Class I histone deacetylases (HDACs 1–3) are essential regulators of gene expression. The enzymes are recruited to chromatin as part of large multi-protein complexes that control the acetylation state of histones and other chromatin-associated factors. In the MiDAC complex, the large ELM2-SANT protein MIDEAS (1045 aa), recruits HDAC1 or 2. In conclusion, our structural and functional studies of the MiDAC complex reveal a striking molecular machine whose architecture appears to have evolved to facilitate processive chromatin deacetylation.

For the tetramer, 63,222 particles were included in the final 4.5-Å map with D2 symmetry applied. The tetrameric complex clearly contains a dimer of the dimeric complexes with no obvious structural perturbations. The arrangement is such that the DNTTIP1 dimerisation domains are symmetrically juxtaposed, but do not directly interact. The two S-shaped dimers are rotated 180° with respect to each other with the four HDAC subunits positioned at the periphery of the tetramer, which results in a striking three-dimensional X-shaped complex. This three-dimensional X-shape of the tetrameric complex positions the active sites of the four HDACs at the extremities of the complex. The tetramerisation interface between the two dimers is mediated by interactions between the SANT domains. Residues Lys849, Tyr874 and Val878 contribute to the interface between the two neighbouring SANT domains. Interestingly, Lys839 and Lys843 appear to be in a position to interact with the inositol phosphate that is bound to the neighbouring dimer, although there is no apparent density for the side chains. This may explain why it was only possible to obtain a high-resolution map of the tetramer in the presence of inositol phosphate (7.7 Å vs 4.5 Å). Given the overall size of the MiDAC complex and the outward-facing HDAC active sites at the complex extremities, it is likely that MiDAC is able to simultaneously target multiple nucleosomes.

>MGATGDAEQPRGPSGAERGGLELGDAGAAGQLVLTNPWNIMIKHRQVQRRGRRSQMTTSFTDPAISMDLLRAVLQPSINEEIQTVFNKYMKFFQKAALNVRDNVGEEVDAEQLIQEACRSCLEQAKLLFS[4x];>[4x]MAQTQGTRRKVCYYYDGDVGNYYYGQGHPMKPHRIRMTHNLLLNYGLYRKMEIYRPHKANAEEMTKYHSDDYIKFLRSIRPDNMSEYSKQMQRFNVGEDCPVFDGLFEFCQLSTGGSVASAVKLNKQQTDIAVNWAGGLHHAKKSEASGFCYVNDIVLAILELLKYHQRVLYIDIDIHHGDGVEEAFYTTDRVMTVSFHKYGEYFPGTGDLRDIGAGKGKYYAVNYPLRDGIDDESYEAIFKPVMSKVMEMFQPSAVVLQCGSDSLSGDRLGCFNLTIKGHAKCVEFVKSFNLPMLMLGGGGYTIRNVARCWTYETAVALDTEIPNELPYNDYFEYFGPDFKLHISPSNMTNQNTNEYLEKIKQRLFENLRMLPHAPGVQMQAIPEDAIPEESGDEDEDDPDKRISICSSDKRIACEEEFSDSEEEGEGGRKNSSNFKKAKRVKTEDEKEKDPEEKKEVTEEEKTKEEKPEAKGVKEEVKLA;>GAVSIEPRINVGSRFQAEIPLMRDRALAAADPHKADLVWQPWEDLESSREKQRQVEDLLTAACSSIFPGAGTNQELALHCLHESRGDILETLNKLLLKKPLRPHNHPLATYHYTGSDQWKMAERKLFNKGIAIYKKDFFLVQKLIQTKTVAQCVEFYYTYKKQVKIGRNGTLT[4x]Pyridaben | C19 H25 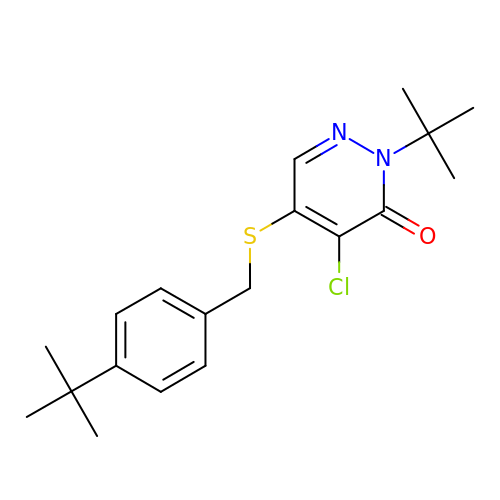Cl N2 O S | DWFZBUWUXWZWKD-UHFFFAOYSA-N Here, we determine mycobacterial MsRv1273c/72c to be an isoniazid efflux pump and determine several structures by cryo-electron microscopy showing specific asymmetrical features including an N-terminal extending loop and a periplasmic helical hairpin only found in MsRv1272c. Thus, MsRv1273c should have a degenerate site impaired for ATPase activity while MsRv1272c has a functional consensus site with the classic enzymatic motifs. Confirmation that this is correct was achieved by mutating both E553Q and D497N, creating the double mutant, which has little activity. Together, these results indicate that the consensus site of MsRv1273c/72c is functional with normal ATPase activity while its degenerate site exhibits very low activity. Thus, MsRv1273c/72c is a drug efflux pump for isoniazid, but not ethambutol.

In another experiment, vanadate (Vi) was added in an attempt to trap the transporter in a conformation immediately after ATP hydrolysis. In such a state, ADP together with vanadate should stabilize the NBD dimer and trap an Occ state. After treatment with ATP and vanadate, the cryo-EM structure of MsRv1273c/72c was solved and showed an ATP | ADP+Vi-bound Occ (Vi) state at 2.7 Å resolution. Since both structures adopt a similar conformation, only the ATP-bound Occ state was analyzed and compared here. In this study, we expected to capture the OF state by using AMPPNP, vanadate or the EtoQ mutant to induce NBD closure. However, the IFasym states and Occ state were observed instead of the OF state. Our results imply that the transporter is more stable at the Occ state than the OF state when the NBDs are fully closed.

> MPEVVGSYFQSNMLWALLRQYVRPYRWLLAVVAVLQVISNMASLYLPTVNAAIIDDGVAKGDTARIVELGAVMLGVTALQVVCAVGAVFFGARAATGFGHDLRAAVFTHVTTFSAEEAGRFGAASLLTRTTNDVGHIQQLVQLTVTMLITAPIMSIGGIFMALHQDAGLSWLLLVSVPVLGLANYWIIRHLMPVFTRMQSLIDGINRVLRDQLSGIRVIRAFAREPLERVRFAEANQTLSDSALEAGRWQALMLPVTTLVINVSSVALIWFGGLRIDAGQMQVGSLIAFLAYFMQILMAVLMATFMLVIFPRAAVCADRIGEVLSTQTAITNPADPVRPAAIAGDIGVHDATFCYPGADRPVLQDVSFTVPRGTTTAVVGSTGSGKSTLISLICRLYDVTSGSLRIDGVDVRDLDIEQLWSAIGLVPQRGYLFSGTVAENLRYGRADATDDEMWEALRVAAAADFVRAHPQGLDMPVAQGGINFSGGQRQRLAIARAVIRRPAIYLFDDAFSALDVHTDARVRDALREVAADATVVIVSQRISTVIEADQVVVIDDGRVVGIGTHDTLLADCPIYAEFAESQALTAGEPR;> MRRGALPQAPLERTRDFKGSAIRLARRLLPQRALTLAVILLGVGGIAIGVIGPRILGHATDLLFNGVIGRELPAGLTKEQAVEAARARGDGTFADLLSGMDIVPGQGVDFGAVGRTLALALGLYLVAALLVWVQARLLNVTVQRTMVALRAEVQEKIHRLPLSYFDSRQRGEVLSRVTNDVDNIQNSVSMTISQLLTSVLTVFAVLVMMLTISPLLTLFTVVTVPASLWVTRWITRRSQPLFVAQWRNTGRLAAHLEETYSGFTIVKTFGHREAAAGKFAELNSETQQSSFGAQFFSGLVSPATMFIGNLSYVAVAVVGGLQVATGQITLGSIQAFIQYVRQFNQPLTQVAGMYNTLQSGIASAERVFDLLDTEEESADSPRRADVRTGRVEFEHVSFSYVPGTPVIEDLSLVAEPGSTVAIVGPTGAGKTTLVNLLMRFYDVDSGRITIDGVDIASVSRESLRASIGMVLQDTWLFAGTIYDNIAYGRPDADEDEVIEAATAAYVDRFVHTLPNGYDTRVDDDGGAISAGEKQLITIARAVLARPKLLVLDEATSSVDTRTELLIAHAMAELRRDRTSFIIAHRLSTIRDADLILVMDSGRIIERGTHEELLARHGRYWEMTRVHLGGIKAFHHHHHHHHHH>[6x]MADFKFEPMRSLIYVDCVSEDYRPKLQRWIYKVHIPDSISQFEPYVTKYAFYPSFPIPPQGDRFGYARMQLTEHHWLVSDLDPRLEIKAIAETFPMDVLVWQGQIPAAAHTDAQIDSDGDAGNAARKSNNAEGNPFIFAFLPMWWEKDLKG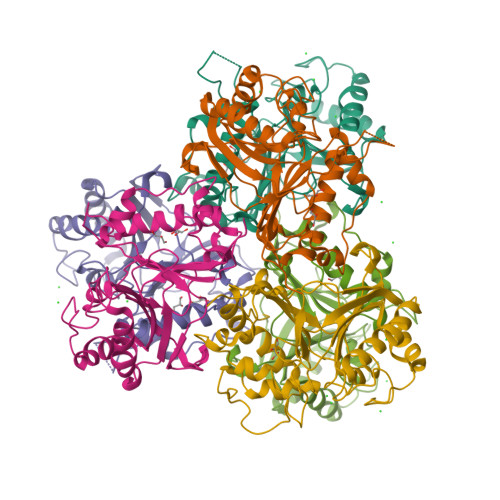KGRTIEDGANYRFNMTIGFPEGVDKAEGEKWLFEKVVPILQAAPECTRVLASAVKKDINGCVMDWVLEIWFENQSGWYKVMVDDMKALEKPSWAQQDAFAFLKPYHNVCSAAVADYTPSNNLANYRGYITMR In response to extracellular stimuli, sphingomyelinases (SMases) remove the phosphocholine head group from sphingomyelin to rapidly generate ceramides. In mammals, nSMases play pivotal roles in ceramide-related signal transduction. SMPD2 was the first mammalian nSMase to be identified and cloned. SMPD2 mainly locates to the endoplasmic reticulum (ER)14 and nuclear matrix, and it requires divalent cations (Mg2+) for activation.

Purified hSMPD2 proteins were subjected to cryo-electron microscopy (cryo-EM) study, and we ultimately obtained a 3.07-Å hSMPD2 structure after sample preparation, images collection and data processing. In contrast to previously reported monomeric SMase structures, hSMPD2 adopts a dimeric architecture with rigorous binary symmetry and with four transmembrane helices (TMHs) protruding into the membrane. In contrast to the density for the TMHs, the densities for the loop preceding TMH1 and for residues 403 − 423 following TMH2 were disordered and were not modeled. hSMPD2 is composed of a transmembrane domain (TMD) and a catalytic domain (CAD) and occupies a spatial volume of approximately 85 × 60 × 80 Å3. Each monomer mainly comprises two TMHs, twelve β-sheets, and four α-helices, forming a special L-shaped architecture (Fig. 1e−f). The dimer interface of hSMPD2 is formed mainly by TMH2 within the TMD and by β6 and α3 within the CAD. Dimeric hSMPD2 is stabilized by substantial hydrophobic interactions and π − π interactions between TMH2 from each protomer. In addition, residue R395 within TMH2 of one protomer interacts with Q91 within the CAD of the other protomer, and residues H164 and K168 from α3 of one protomer interact with E92 from β6 of the neighboring protomer. In the TMD interface, we also observed densities within the hydrophobic cleft, which we attributed to four acyl chains that interact extensively with residues F371, L373, and F374 within TMH2 and with residues P104, Y105, W112, and F113 within the CAD of both protomers (Fig. 2b and Supplementary Figs. 7a−b). The presence of these hydrophobic lipids contributes to the stabilization of dimeric hSMPD2. In our current hSMPD2 structure, we observed a magnesium ion located in a negatively charged cleft in the CAD that is further coordinated by residues N15 and E49 in the active site. Akin to the reported homologous nSMase structures, the current hSMPD2 structure represents a substrate binding groove exposed state, that is ready to bind and hydrolysis substrates.

>[2x]MKPNFSLRLRIFNLNCWGIPYLSKHRADRMRRLGDFLNQESFDLALLEEVWSEQDFQYLRQKLSPTYPAAHHFRSGIIGSGLCVFSKHPIQELTQHIYTLNGYPYMIHHGDWFSGKAVGLLVLHLSGMVLNAYVTHLHAEYNRQKDIYLAHRVAQAWELAQFIHHTSKKADVVLLCGDLNMHPEDLGCCLLKEWTGLHDAYLETRDFKGSEEGNTMVPKNCYVSQQELKPFPFGVRIDYVLYKAVSGFYISCKSFETTTGFDPHRGTPLSDHEALMATLFVRHSPPQQNPSSTHGPAERSPLMCVLKEAWTELGLGMAQARWWATFASYVIGLGLLLLALLCVLAAGGGAGEAAILLWTPSVGLVLWAGAFYLFHVQEVNGLYRAQAELQHVLGRAREAQDLGPEPQPALLLGQQEGDRTKEQ> MHHHHHHSSGRENLYFQGMTRDFKPGDLIFAKMKGYPHWPARVDEVPDGAVKPPTNKLPIFFFGTHETAFLGPKDIFPYSENKEKYGK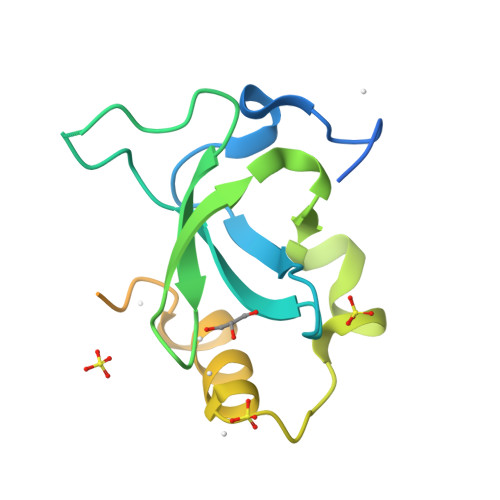PNKRKGFNEGLWEIDNNPKVKFSSQQAATKQSNASSDVEVEEKETSVSKEDTDHEEKASNEDVTK>[4x]MAAKNAFYAQSGGVTAVINASAAGVIEAARKQSGKIGRIYAGRNGIIGALTEDLIDTGQESDAAISALRYTPSGAFGSCRYKLKSLEQNRREYERLIEVFKAHDIGYFFYNGGGDSADTCLKVSQLSGTLGYPIQAIHVPKTVDNDLPITDCCPGFGSVAKYIAVSTLEASFDVASMSATSTKVFVLEVMGRHAGWIAAAGGLASSPEREIPVVILFPEISFDKQKFLAKVDSCVKKFGY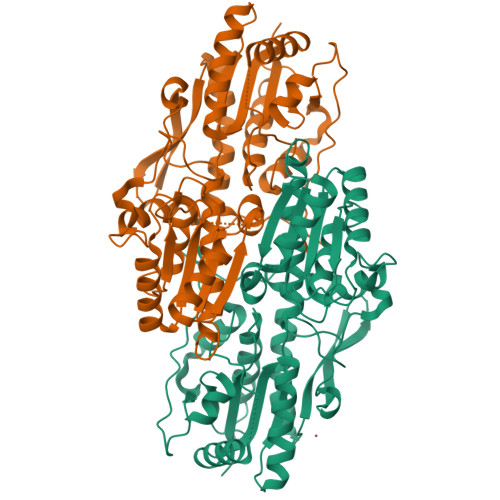CSVVVSEGVKGDDGKFLSDQGVRDAFGHAQLGGVAPVVASMVKEGLGLKYHWGVADYLQRAARHIASKTDVEQAYAMGQAAVEFAVQGHNSVMPTIERISARPYQWKVGMAQLSQVANVEKMMPENFITEDGFGITDLCREYLAPLIEGEDYPPYKDGLPDYVRLKNVAVPKKLSGFTL>[3x]MDDCSGKT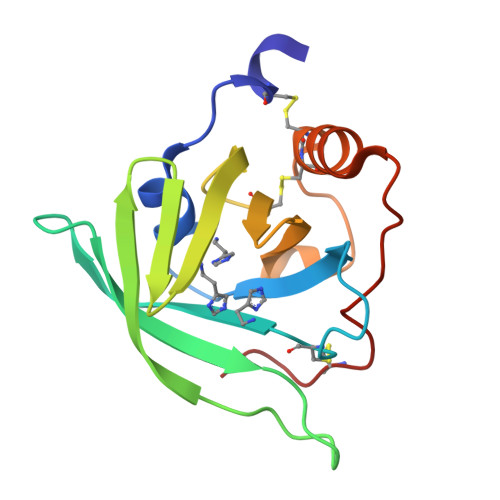DAWTSIKGPKTGGYWLKQTTKTGENECTYVKGTDFKENTKTATYTYGYKDASGKLTKTTGTATAKGSDIVVGSDTSTVIYTDGKTCDVVKHGGHTELWVHSSKTSGGYNNCCDKKFTETRGSTPANEVYKKCPGMP> MGGSHHHHHHSRAWRHPQGGSHHHHHHGMRDLYDDDDKDPPEISPHAPASADATRIAA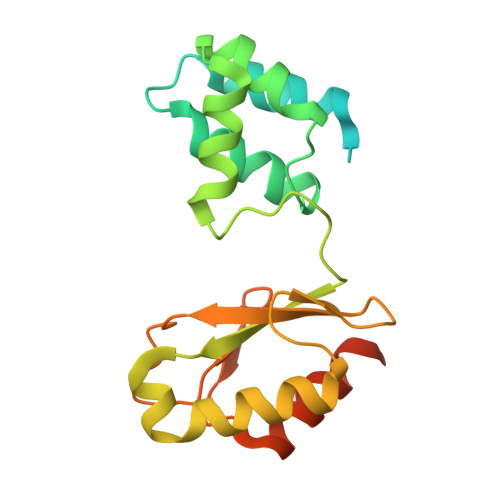IVAARQDIPGALLPILHEIQDTQGYIPDAAVPVIARALNLSRAEVHGVITFYHHFRQQPAGRHVVQVCRAEACQSVGAEALAEHAQRALGCGFHETTADGQVTLEPVYCLGQCACGPAVMVGEQLHGYVDARRFDALVRSLRESSAEKTTEAAEAQA Hemoglobins (Hbs) are iron-protoporphyrin-IX (heme b)-binding proteins that are found in all kingdoms of life. In all functional globins, an invariant His residue forms a coordinate bond to the central Fe atom at the proximal site of the heme cofactor, whereas substrates bind to the sixth coordination site of the Fe ion, located at the distal site. The aim of this study was to obtain structural information on a ferrous pentacoordinate Chlamydomonas 2/2Hb, THB11 (gene ID Cre16.g662750), which is one of the algal Hbs that feature extended N- and, particularly, C-termini of yet unknown function. Here, we report the first crystal structure of a Chlamydomonas pentacoordinate 2/2Hb, the heme-binding domain (HBD) of Chlamydomonas THB11 in its cyanomet form.

We attempted to crystallize all THB11 length variants, however, despite extended screenings for suitable crystallization conditions, only THB11-NC, which is reduced to the heme-binding domain (HBD), and from which the Strep-tag had been removed, formed crystals. THB11-NC crystallized in space group P21 21 21, with one molecule in the crystallographic asymmetric unit. The tertiary structure recapitulates the typical 2/2Hb fold, but unusual features are observed, such as a kink in helix E, a tilted heme plane and a tunnel system possibly shielded by Met residues. Only one heme orientation isomer could be fitted into the electron density map of THB11-NC, and the porphyrin ring is rotated by 180° along the α–γ axis compared to those of THB1, LI637 and Synechocystis or M. tuberculosis GlbN. Normal-coordinate structural decomposition analysis indicates that the heme group of THB11-NC features an overall out of plane displacement of 0.49 Å, and the heme distortions are dominated by doming and ruffling. The imidazole ring of THB11-NC HisF8(81) (note that residues are indicated in the Perutz nomenclature, followed by their numbers in the structure in brackets) is in a moderately staggered position, and its plane is tilted towards the heme group. In the distal site of THB11-NC, the CN– ligand lies in moderate H-bond distance to the hydroxyl group of TyrB10(32) (2.8 Å), whereas position E7 is occupied by Leu53, and the distance of the ligand to the amide group of GlnE11(57) is 3.9 Å (N atom) or 4.9 Å (O atom). LysE10(56) points away from the heme cofactor, being located at the E helix side that is averted from the distal niche. In the THB11-NC structure, MetH11(123) as well as the adjacent LeuH12(124) were modeled in two conformations, and, together with MetG9(99), MetH11(123) restricts the site at which the ST exits in M. tuberculosis GlbN. According to the calibration of the SEC column, these represented approximately tri- and heptamers in case of THB11 and THB11-N, and mono- and trimers in case of THB11-C, whereas the elution volume of the single THB11-NC peak corresponded to a monomer.

> GSAGTSTATNAGPLLQRVGGLDVVKKVVELFYRKLYADPQLIKYLHDQDPMHLRAKQSMFVSWLFGPPNVPYTGKSVRIAHLRIIKQRGFSPEDFDLGMKYFEEAMTELGAPEVLRGEVMRRMLPYKDAIFTPAAGDAAEEA>AIDEIKSRGYLLVGLSADFPPFEFVDENGNIVGFDVDLAKEIARRLGVELKIVDMTFDGLIPSLLTKKIDVIISGMTITEERKKVVAFSDPYFDAGQVIVVRKDSDFRPKTYEDLVGKTVAVQIGTTGDIEVSKY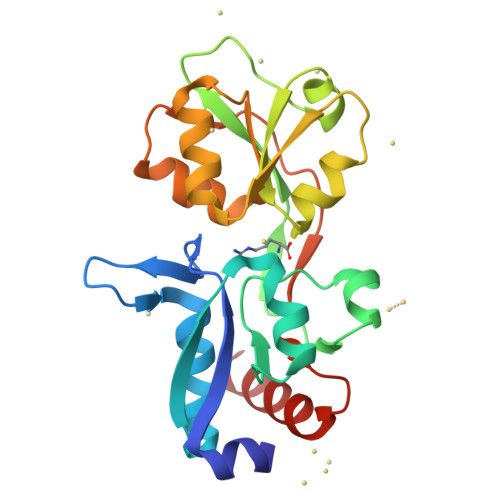DGIKVVRFDKFTDAFLELKRGRADAVVLDSATARAFVAKNPDLVISSGVLSSEQYGIAVRKEDTDLLEFINSVLRELK[2x]> GPLGSMTNINFSALLRGERMCPLTREIHSQMLIVTKSYSLVETFRAFPR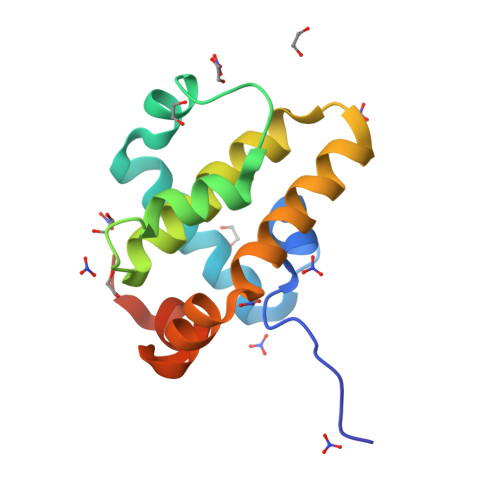LPNILEIGNNIVSDGNLNWGRILILLGISQLYFTKSESESERTQITEQLERFFRQDAISNWIASNGGWVTCASLDLRNYSSVT>MGLWFEEGAEERQVLGPFREFLKAEVAPGAAERDRTGAFPWDLVRKLAEFGVFGALVPEAYGGAGLSTRLFARMVEAIAYYDGALALTVASHNSLATGHILLAGSEAQKEAFLPKLASGEALGAWGLTEPGSGSDAAALKTKAEKVEGGWRLNGTKQFITQGSVAGVYVVMARTDPPPSPERKHQGISAFAFFRPERGLKVGRKEEKLGLTASDTAQLILEDLFVPEEALLGERGKGFYDVLRVLDGGRIGIAAMAVGLGQAALDYAL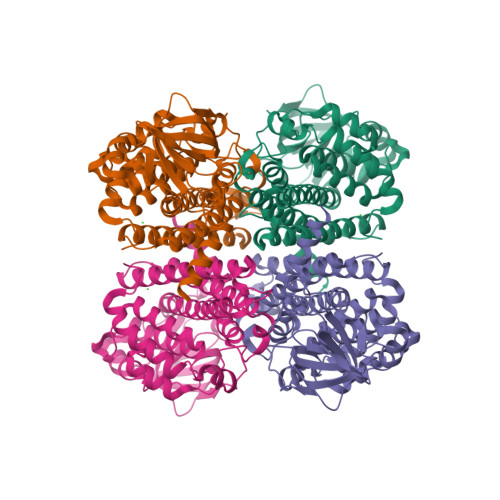AYAKGREAFGRPIAEFEGVSFKLAEAATELEAARLLYLKAAELKDAGRPFTLEAAQAKLFASEAAVKACDEAIQILGGYGYVKDYPVERYWRDARLTRIGEGTSEILKLVIARRLLEAV[4x]> GSQEQKGDAPTCGICHKTKFADGCGHN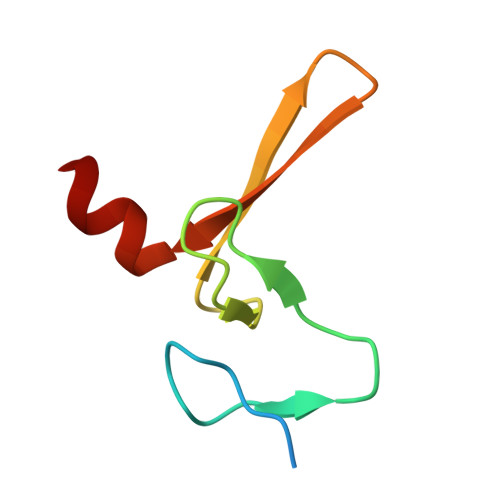CSYCQTKFCARCGGRVSLRSNKVMWVCNLCRKQQE>MGSDKIHHHHHHMAILNILEFPDPRLRTIAKPVEVVDDAVRQLIDDMFETMYEAPGIGLAATQVNVHKRIVVMDLSEDKSEPRVFINPEFEPLTEEMDQYQEGCLSVPGFYENVDRPQKVRIKALDRDGNPFEEV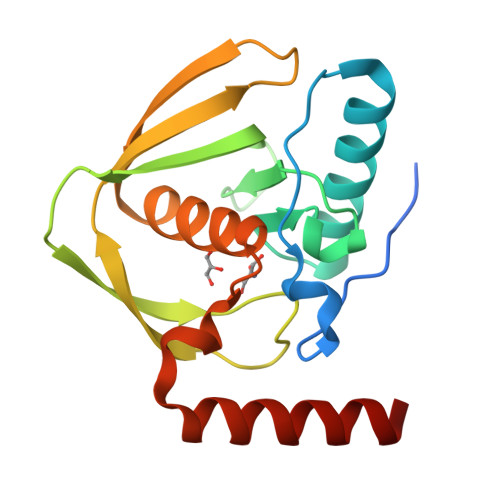AEGLLAVCIQHECDHLNGKLFVDYLSTLKRDRIRKKLEKQHRQQA[2x]> ANGTSSAFTQVDNFSHFYDRGNHLVNGKPSFTVDQAADQLTRSGASWYDLNGDGVINLSYTFLTSPPPGYASRGLGTFSSFSGLQKEQAKLSLESWADVAKVTFTEGPAARGDDGHMTFANFSASNGGAAFAYLPNSSRKGESWYLINKDYDVNKTPGEGNYGRQTLTHEIGHTLGLSHPGDYNAGNGNPSYRDAVYGEDTRAYSVMSYWSEKNTGQVFTKTGEGAYASAPLLDDIAAVQKLYGANMETRAGDTVYGFNSTADRDYYSATSATDKLIFSVWDGGGNDTLDFSGFSQNQKINLAAGSFSDVGGMTGNVSIAQGVTIENAIGGSGNDLLLGNAASNILKGGAGNDIIYGGGGADKLWGGSGSDTFVYREVSDSTPKAADTLMDFQTGLDKIDLTGITHLSGLNFVNAFTGQAGDAVVSYN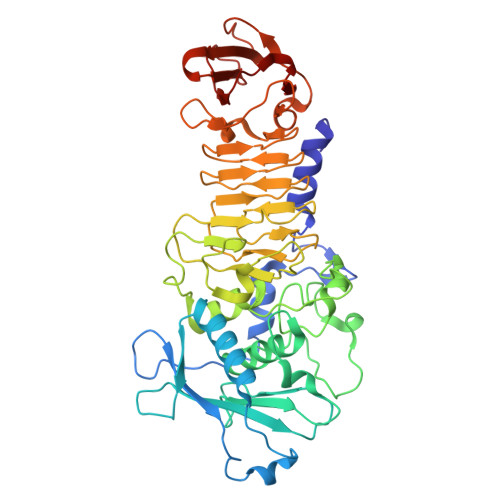QASNAGSLQVDFSGHGVADFLITTVGQVATYDIVA>[12x]MNQELKLRPLEREDLKFVHELNNNAHIMSYWFEEPYEAFVELQDLYDKHIHDQSERRFIVEKDNEMVG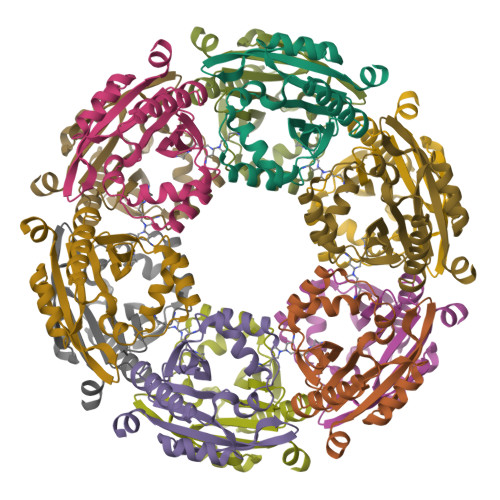LVELVEIDYIHRRTEFQIIIDPNYQGYGYAVDATRLAMDYAFSVLNMHKIYLVVDKENEKAVHVYKKVGFMVEGELIDEFFVDGNYHNAIRMCMFQKQYFENK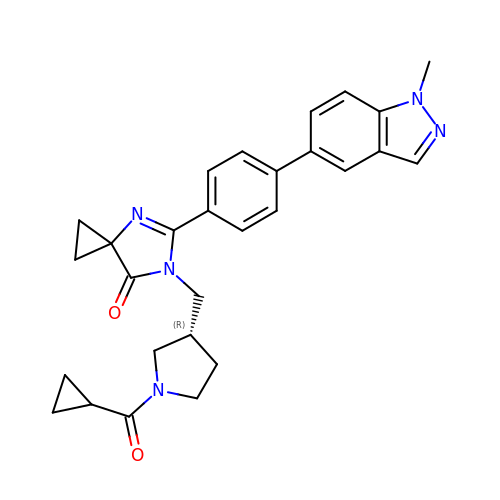6-{[(3R)-1-(cyclopropylcarbonyl)pyrrolidin-3-yl]methyl}-5-[4-(1-methyl-1H-indazol-5-yl)phenyl]-4,6-diazaspiro[2.4]hept-4-en-7-one | C28 H29 N5 O2 | KYFZEWZCYBWMGN-GOSISDBHSA-N5-[(6-bromo-1H-indol-1-yl)methyl]-2-methylfuran-3-carboxylic 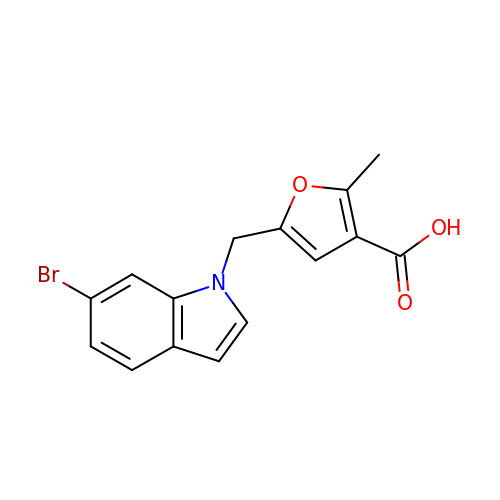acid | C15 H12 Br N O3 | XCOVJISMCVGULK-UHFFFAOYSA-N> MYQQDQVVKEDNIEAVGKKLHEYNTQFQEKSREYDRLYEDYTRTSQEIQMKRTAIEAFNETIKIFEEQCQTQERYSKEYIEKFKREGNETEIQRIMHNYEKLKSRISEIVDSRRRLEEDLKKQAAEYREIDKRMNSIKPDLIQLRKTRDQYLMW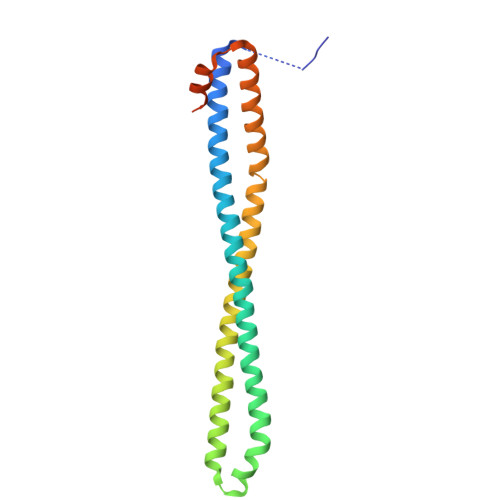LTQKGVRQKKLNEWLGNSRACSLEACGTKLVEKY>MATNGMRPIHPGEILRDEFLMEFDISPAALARALKVSAPTVNDIVREQRGISADMAIRLGRYFDTSAQ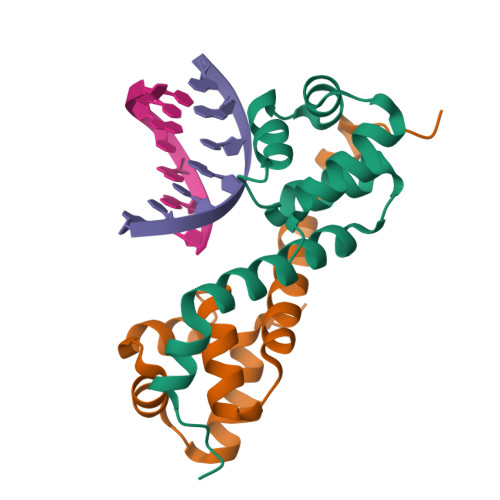FWMNLQSEYSLATAYAANGKQIEHEIEPLLAHG[2x]>[2x]MEWSQIFHDITTKHDFKAMHDFLEKEYSTAIVYPDRENIYQAFDLTPFENIKVVILGQDPYHGPNQAHGLAFSVQPNAKFPPSLRNMYKELADDIGCVRQTPHLQDWAREGVLLLNTVLTVRQGEANSHRDIGWETFTDEIIKAVSDYKEHVVFILWGKPAQQKIKLIDTSKHCIIKSVHPSPLSAYRGFFGSKPYSKANTYLESVGKSPINWCESEALEHHHHHH;>[2x]MYKNIEDLNKFA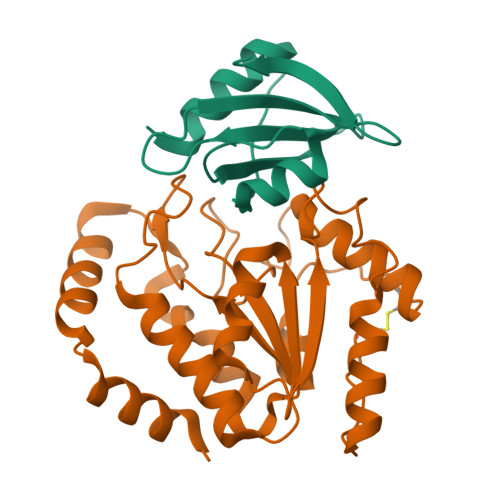SKILETEISFEESITFTPDEVEENIGEKPNRDKICHSTSLEDGRVIMLLTELEPNYTPWKLLELEEDGFKELYSKSI>[2x]REVLTGGHSVSAPQENRIYVMDSVFMHLTESRVHVYDYTNGKFLGMVPTAFNGHVQVSNDGKKIYTMTTYHERITRGKRSDVVEVWDADKLTFEKEISLPPKRVQGLNYDGLFRQTTDGKFIVLQNASPATSIGIVDVAKGDYVEDVTAAAGCWSVIPQP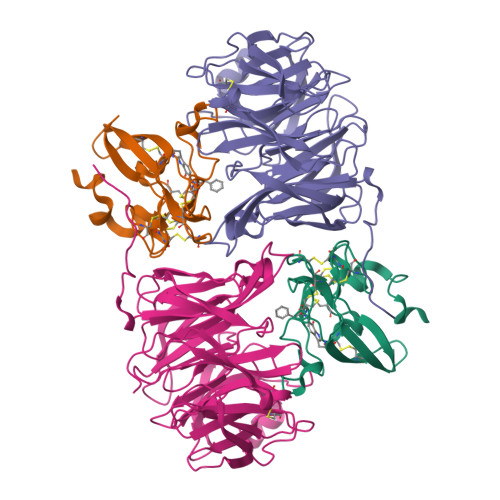NRPRSFMTICGDGGLLTINLGEDGKVASQSRSKQMFSVKDDPIFIAPALDKDKAHFVSYYGNVYSADFSGDEVKVDGPWSLLNDEDKAKNWVPGGYNLVGLHRASGRMYVFMHPDGKEGTHKFPAAEIWVMDTKTKQRVARIPGRDALSMTIDQQRNLMLTLDGGNVNVYDISQPEPKLLRTIEGAAEASLQVQFHPVGGT;>[2x]HISLNPDLANEDEVNSCDYWRHCAVDGFLCSCCGGTTTTCPPGSTPSPISWIGTCHNPHDGKDYLISYHDCCGKTACGRCQCNTQTRERPGYEFFLHNDVNWCMANENSTFHCTTSVLVGLA InsP3 3-kinase, a highly specific enzyme binding InsP3 in just one mode, phosphorylates InsP3 specifically at its secondary 3-hydroxyl group to generate a tetrakisphosphate. The structure of the IP3K kinase domain (IP3K-KD) revealed that the inositol polyphosphate kinase (IPK) family conserves the protein kinase (PK) fold organization in two lobes, the N- and C-lobes, binding the ATP in between them in a similar way. However, they present a third lobe, the IP-lobe inserted into the C-lobe, which accounts for most of the interactions with the inositide substrate. Summarizing, IP3K substrate recognition entails close interactions with the three phosphates in positions 1, 4 and 5 of the InsP or of the corresponding carbohydrate-based analogues.

We found that l-scyllo-1,2,4-trisphosphate (1-s) is a good IP3K substrate. In further support, the crystal structures in complex with substrate 1-s and its putative product, the synthetic symmetrical scyllo-inositol 1,2,3,5-tetrakisphosphate (1-p, in this study, equivalent to natural InsP4 in myo-inositol polyphosphate regiochemistry), show that they both perfectly mimic InsP3 and InsP4 binding. The main difference is the shift from the InsP3 site in the scyllo-derived compounds. This shift causes a distance increase between the Pγ of ATP and the pseudo 3-OH of the inositol substrate by more than 1 Å (from 4.6 Å in the InsP3 complex to 5.8 Å in that for 1-s). We observe that the scyllo analogues of InsP3 and InsP4 (1-s and 1-p) with an inverted pseudo 2-OH group (therefore with all substituents equatorial) are better ligands for IP3K than the natural ones, exhibiting IC50 values of 36 nM and 51 nM respectively, compared to a value of 140 nM for InsP3. In this work, the identification of unusual substrates (InsP3 and compounds 1-s, 5-s, 6a–s and 7a–s) that expand the reaction center’s distance from 4.6 Å (InsP3) to a range of 3.8–5.8 Å suggests that IP3K phosphorylates a range of substrates possibly with a strong contribution of a dissociative mechanism.

>[2x]GSHMSWVQLAGHTGSFKAAGTSGLILKRCSEPERYCLARLMADALRGCVPAFHGVVERDGESYLQLQDLLDGFDGPCVLDCKMGVRTYLEEELTKARERPKLRKDMYKKMLAVDPEAPTEEEHAQRAVTKPRYMQWREGISSSTTLGFRIEGIKKADGSCSTDFKTTRSREQVLRVFEEFVQGDEEVLRRYLNRLQQIRDTLEVSEFFRRHEVIGSSLLFVHDHCHRAGVWLIDFGKTTPLPDGQILDHRRPWEEGNREDGYLLGLDNLIGILASLAER> PQAGSLDLQIDEEQPAGTLIGDISAGLPAGTAAPLMYFISAQEGSGVGTDLAIDEHSGVVRTARVLDREQRDRYRFTAVTPDGATVEVTVRVADINDHAPAFPQARAALQVPEHTAFGTRYPLEPARDADAGRLGTQGYALSGDGAGETFRLETRPGPDGTPVPELVV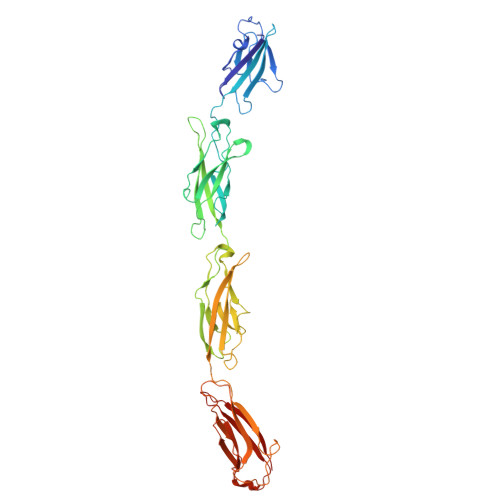TGELDRENRSHYMLQLEAYDGGSPPRRAQALLDVTLLDINDHAPAFNQSRYHAVVSESLAPGSPVLQVFASDADAGVNGAVTYEINRRQSEGDGPFSIDAHTGLLQLERPLDFEQRRVHELVVQARDGGAHPELGSAFVTVHVRDANDNQPSMTVIFLSADGSPQVSEAAPPGQLVARISVSDPDDGDFAHVNVSLEGGEGHFALSTQDSVIYLVCVARRLDREERDAYNLRVTATDSGSPPLRAEAAFVLHV In this study, we characterized a thermostable endochitinase (Chi23) that can hydrolyze both crystalline and colloidal chitin. Chi23, from a marine bacterium Pseudoalteromonas aurantia DSM6057, is a member of the subfamily B of the GH18 family. However, different from other modular endochitinases of the subfamily B, Chi23 is a single-domain enzyme containing only a catalytic domain. The catalytic domains (CaD) of GH18 chitinases adopt the classical (β/α)8 TIM-barrel fold with a conserved catalytic DxDxE motif.

The crystal of Chi23 belongs to the P121 space group with four molecules loosely packed per asymmetric unit. Gel filtration analysis showed that Chi23 presents as monomers in solution. Consistent with sequence analysis, structural analysis also showed that Chi23 is a single-domain protein containing only a CaD, which is distinct from other endochitinases of the GH18 subfamily B that are all modular proteins. Chi23 comprises 14 α-helices and 10 β-sheets. The catalytic 113DxDxE117 motif is located in the loop between β6 and α5, and a hydrogen bond is formed between the catalytic residues Asp115 and Glu117. For Chi23, it only has such an α-helix, and lacks the β-sheets for the formation of a β-hairpin subdomain. Therefore, different from other bacterial chitinases from the GH18 subfamily B, Chi23 does not have a β-hairpin subdomain. However, similar to PPL2, Chi23 only has extremely short loops in these corresponding regions. Moreover, surface residues Phe30-Ser44 in Chi23 form two antiparallel β-sheets, which are conserved in nearly all eukaryotic chitinases of the GH18 subfamily B, but not in the bacterial chitinases of this subfamily where only one or no corresponding β-sheet is formed. A detailed structural analysis of Chi23 showed that the side chain of Asp229 forms four hydrogen bonds with the solvent-exposed residues Thr226 and Ser264, and that the side chain of Gln261 is hydrogen bonded to residues Ser10 and Asn9 lining on the substrate cleft surface.

>MSKTITYYNSGAVPLINASELPYDVVNLAFLSSSSNNPFNLVLSGAIAATESSFTTNTIEAIKVMQHKGQKVLISFGGGTMGSNAYRSLSEDTAKLADSLASFVKNNQLDGVDIDYEDTAAFTGQAGYDGAQFLISLTQELRKRLPSPDYIISHAPQPPYLEQGGYMAGYVEVVELVGQEIDWLNVQFYNNPPWSANPDQIVSSYLNYTKLPNMSPEKVIAGFPVTQNDAGSGYMPVQTIINEVIKPIQQQSSLGGIMNWQFSSDHNGDWIKAIAQSLNSLEHHHHHH[4x]>TRRTAFFFDELCLWHAAGPHALTLPVGGWVQPPAAAGHAESPETKRRLKSLLDVSGLTARLQLRSAPPASDEDLLRVHPAHYLERFKALSDAGGGSLGQDAPIGPGSYEIARLSAGLAIAALDAVLAGEADNAYSLSRPPGHHCLPDQAMGFCFFANIAVAIEAAKARHGVERVAVLDWDVHHGNGTQAIYYRRDDVLSISLHQDGCFPPGYSGAEDIGEDRGRGFNLNVPLLPGGGHDAYMQAMQRIVLPALERFRPQLIVVASGFDANAVDPLARMQLHSDSFRAMTAMVRDAAERHAGGRLVVVHEGGFSEAYVPFCGLAVIEELSGVRSA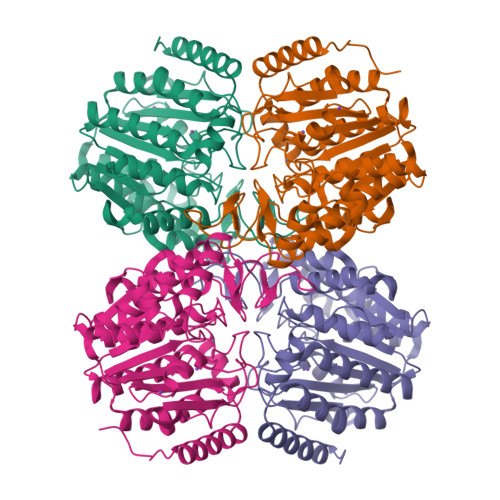VRDPLRDFIELQQPNAAFRDFQRQRLEELAAQFGLCPAQPLQAAR[2x]>[2x]SNAMETLNDIKKILINVGLYQGFDLTDPKVSEEVNHETANMKWIKDYTSDGNWDNEFKEDLKNFLDYMEVCQLALNDKNFKIASNSLFMAMIYAGNLSLIFDSIKTDISTLLSAE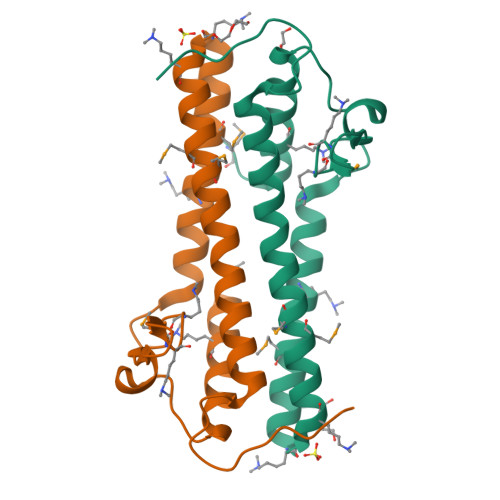YKKNSFSWPSLDE> HPTNVQRLAEPSQMLKHAVVNLINYQ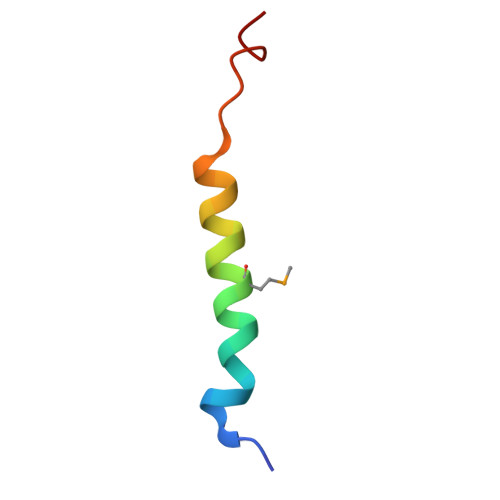DDAELA> MPYIEKLELKGFKSYGNKKVVIPFSKGFTAIVGANGSGKSNIGDAILFVLGGLSAKAMRASRISDLIFAGSKNEPPAKYAEVAIYFNNEDRGFPIDEDEVVIRRRVYPDGRSSYWLNGRRATRSEILDILTAAMISPDGYNIVLQGDITKFIKMSPLERRLLIDD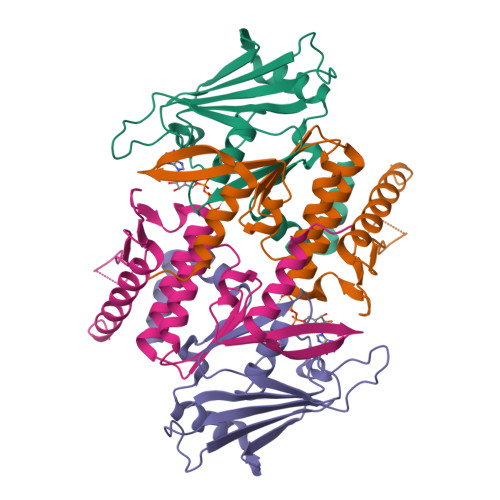ISGIAEYDSKKEKALEE;> EKEKKNVFMRTFEAISRNFSEIFAKLSPGGSARLILENPEDPFSGGLEIEAKPAGKDVKRIEAMSGGEKALTALAFVFAIQKFKPAPFYLFDQIDAHLDDANVKRVADLIKESSKESQFIVITLRDVMMANADKIIGVSMRDGVSKVVSLSLEKAMKILEEIRKKQGWEHGN>[4x]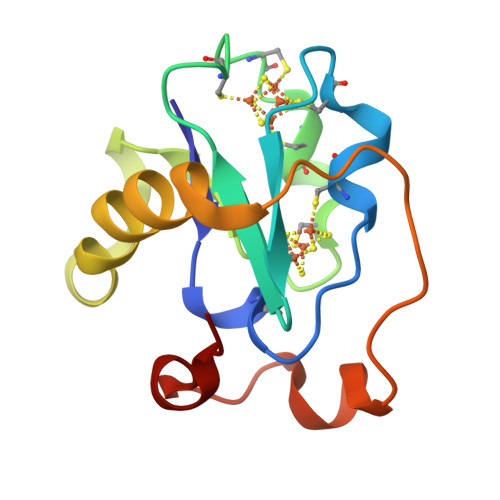AFVVTDNCIKCKYTDCVEVCPVDCFYEGPNFLVIHPDECNDCALCEPECPAQAIFSEDEVPEDMQEFIQLNAELAEVWPNITEKKDPLPDAEDWDGVKGKLQHLER Bacterial caseinolytic protease P subunit (ClpP) is important and vital for cell survival and infectivity. The caseinolytic protease P (ClpP) subunit is a compartmentalized structure with two stacked heptameric rings that form a central chamber containing 14 identical catalytic sites sequestered by two protective axial pores. In any case, even the degradation of small oligopeptides depends on some structural factors, and the most important one is the orientation and positioning of the catalytic triads formed by Ser98, His123, and Asp17224. The protein’s mode of action corresponds to that of a chymotrypsin-like protease, and it is described in two main steps: acylation and deacylation.

However, when the same assays are performed with a SeClpP sample supplemented with 20% w/v glycerol, an increase in peptidolytic activity is not observed. This simple triol is known as chemical chaperone and protein stabilizer, and if used in cell lysis and purification steps, the ClpP sample becomes homogenized with a higher concentration of extended tetradecamers, as noticeable during size-exclusion chromatography, where only one peak is observed. Conversely, glycerol revokes the positive cooperativity, since it stabilizes the tetradecameric SeClpP, also organizing the binding channels.

>[14x]MNLIPTVIETTNRGERAYDIYSRLLKDRIIMLGSQIDDNVANSIVSQLLFLQAQDSEKDIYLYINSPGGSVTAGFAIYDTIQHIKPDVQTICIGMAASMGSFLLAAGAKGKRFALPNAEVMIHQPLGGAQGQATEIEIAANHILKTREKLNRILSERTGQSIEKIQQDTDRDNFLTAAEAKEYGLIDEVMEPEHHHHHH>VSRYVPDMGDLIWVDFDPTKGSEQAGHRPAVVLSPFMYNNKTGMCLCVPCTTQSKGYPFEVVLSGQERDGVALADQVKSIAWRARGATKKGTVAPEELQLIKAKINVLIG[2x];> GPHMIHSSVKRWGNSPAVRIPATLMQALNLNIDDEVKIDLVDGKLIIEPVRKEPVFTLAELVNDI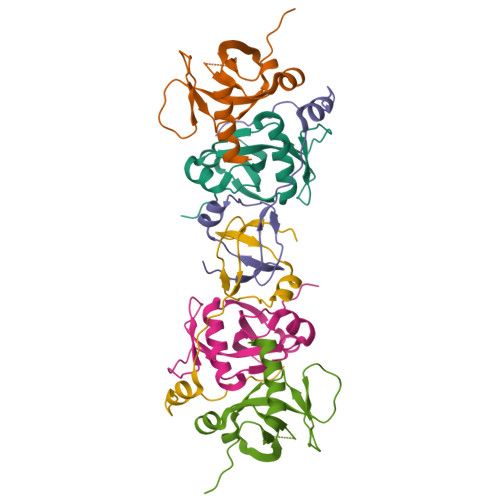TPENLHENIDWGEPKDKEVW>[2x]MISDSMTVEEIRLHLGLALKEKDFVVDK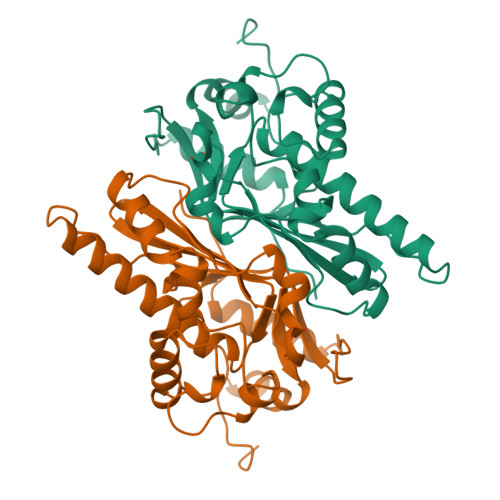TGVKTIEIIGASFVADEPFIFGALNDEYIQRELEWYKSKSLFVKDIPGETPKIWQQVASSKGEINSNYGWAIWSEDNYAQYDMCLAELGQNPDSRRGIMIYTRPSMQFDYNKDGMSDFMCTNTVQYLIRDKKINAVVNMRSNDVVFGFRNDYAWQKYVLDKLVSDLNAGDSTRQYKAGSIIWNVGSLHVYSRHFYLVDHWWKTGETHISKKDYVGKYA>MAHHHHHHENLFYQGPLTPADVHNVAFSKPPIGKRGYNEDEVDAFLDLVENELTR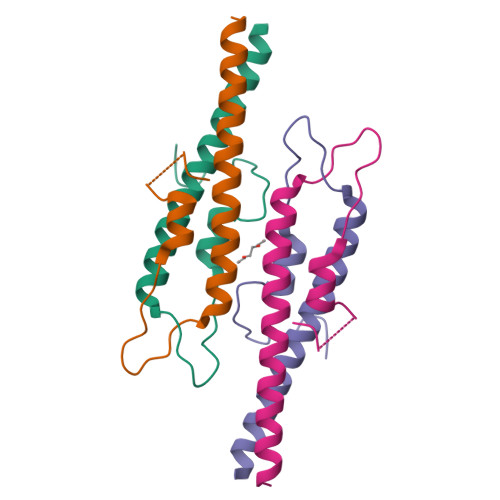LIEENSDLRQRINELDQEL[2x]>[2x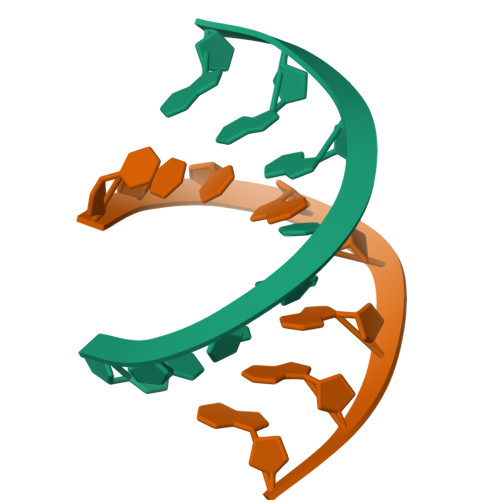]CCCGCGGG>MAKNRRDRNSWGGFSEKTYEWSSEEEEPVKKAGPVQVLIVKDDHSFELDETALNRILLSEAVRDKEVVAVSVAGAFRKGKSFLMDFMLRYMYNQESVDWVGDYNEPLTGFSWRGGSERETTGIQIWSEIFLINKPDGKKVAVLLMDTQGTFDSQSTLRDSATVFALSTMISSIQVYNLSQNVQEDDLQHLQLFTEYGRLAMEETFLKPFQSLIFLVRDWSFPYEFSYGADGGAKFLEKRLKVSGNQHEELQNVRKHIHSCFTNISCFLLPHPGLKVATNPNFDGKLKEIDDEFIKNLKILIPWLLSPESLDIKEINGNKITCRGLVEYFKAYIKIYQGEELPHPKSMLQATAEANNLAAVATAKDTYNKKMEEICGGDKPFLAPNDLQTKHLQLKEESVKLFRGVKKMGGEEFSRRNYLQQLESEIDELYIQYIKHNDSKNIFHAARAAALEHHHHHH[2x]

The ATL1 protein belongs to the dynamin superfamily, members of which comprise a canonical, large GTPase (G) domain, and function in a variety of cellular pathways including vesicle fission, remodeling of organelle membranes, and immunity through antiviral activity. ATL1 is a resident ER enzyme, residing in the high-curvature tubules of the smooth ER, where it tethers and fuses tubules following GTPase-driven reaction cycles to generate and maintain the ER’s polygonal morphology. The N-terminus of ATL1 is composed of the canonical large G domain followed by a flexible linker region and middle domain, facing the cytoplasm, followed by a short, membrane-associated wedge motif with preference for high-curvature ER tubules. Having established a pronounced cellular phenotype, we set out to characterize the effect of the ATL1 N417ins mutation on the protein’s molecular mechanism. It has been established that the N-terminal soluble module of ATL1 consisting of the conserved G and middle domains, which we refer to as the catalytic core, is sufficient to carry out GTP hydrolysis and nucleotide-dependent oligomerization.

Here we present a case of an early onset, complex HSP caused by a novel ATL1 mutation, where an asparagine residue is inserted into the middle domain between arginine residue 416 and tyrosine residue 417 (N417ins), the first reported clinical case caused by a whole codon insertion in ATL1. The protein with the insertion mutation crystallized in the presence of the transition state analog GDP•AlF4− and Mg2+, diffracting to a resolution of 1.9 Å. The structure was solved by molecular replacement in space group P212121 using isolated G and middle domain fragments as the search models, identifying two molecules in the asymmetric unit. The novel, dimeric structure aligns with that of a corresponding ATL1 WT protein bound to GDP•AlF4− (25) with an rmsd value of 0.386 Å, both structures depicting a tight crossover dimer of ATL1’s catalytic core. The inserted N417 residue is surface exposed within the middle domain’s third helix. In this state, the ⍺-helical rung containing the insertion accommodates the additional residue by bulging out slightly, resulting in minimal long-range structural changes. According to the DSSP secondary structure assignment, the inserted residue results in formation of π-helix from residues 415 to 419 (50, 51). The primary variation between WT and insertion-mutant structures lies within the middle domain dimer, where a slight translation is observed toward the second protomer’s middle domain within the dimeric assembly of the mutant, with the middle domain interface tightening by ∼0.7 to 1.2 Å (interface-proximal) to 1.0 to 1.6 Å (solvent-proximal). The only exception to this observed domain translation is residue R416, directly preceding the insertion mutation, which shifts 3.6 Å in its C⍺ position and rotates outward.> MEKGDTHILVFPFPSQGHINPLLQLSKRLIAKGIKVSLVTTLHVSNHLQLQGAYSNSVKIEVISDGSEDRLETDTMRQTLDRFRQKMTKNLEDFLQKAMVSSNPPKFILYDSTMPWVLEVAKEFGLDRAPFYTQSCALNSINYHVLHGQLKLPPETPTISLPSMPLLRPSDLPAYDFDPASTDTIIDLLTSQYS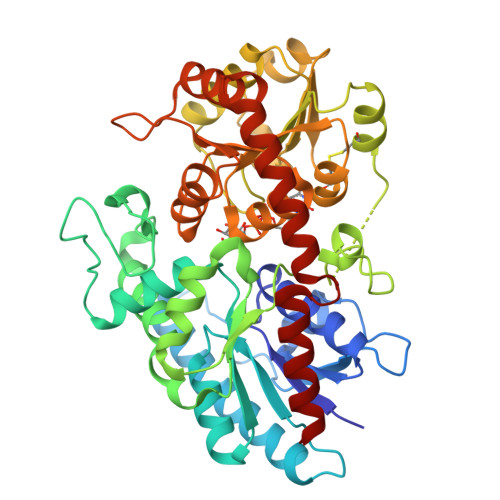NIQDANLLFCNTFDKLEGEIIQWMETLGRPVKTVGPTVPSAYLDKRVENDKHYGLSLFKPNEDVCLKWLDSKPSGSVLYVSYGSLVEMGEEQLKELALGIKETGKFFLWVVRDTEAEKLPPNFVESVAEKGLVVSWCSQLEVLAHPSVGCFFTHCGWNSTLEALCLGVPVVAFPQWADQVTNAKFLEDVWKVGKRVKRNEQRLASKEEVRSCIWEVMEGERASEFKSNSMEWKKWAKEAVDEGGSSDKNIEEFVAMLKQT> KSLKGSRTEKNILTAFAGESQARNRYNYFGGQAKKDGFVQISDIFAETADQEREHAKRLFKFLEGGDLEIVAAFPAGIIADT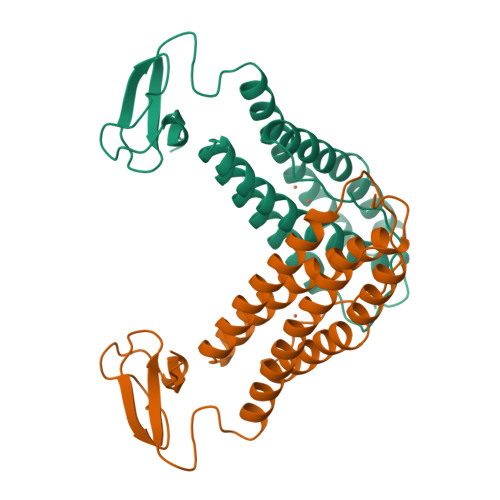HANLIASAAGEHHEYTEMYPSFARIAREEGYEEIARVFASIAVAEEFHEKRFLDFARNIKEGRVFLREQATKWRCRNCGYVHEGTGAPELCPACAHPKAHFELLGINW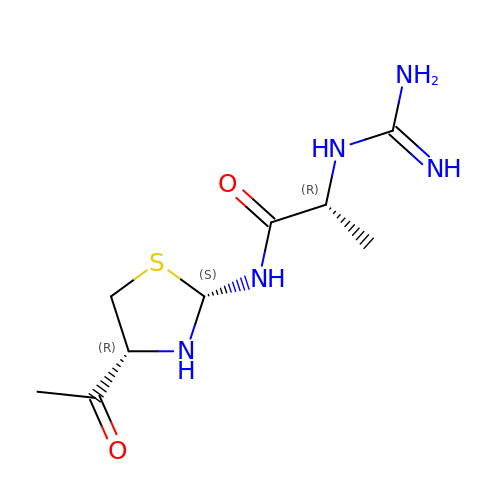(2~{R})-2-carbamimidamido-~{N}-(4-ethanoyl-1,3-thiazolidin-2-yl)propanamide | C9 H17 N5 O2 S | LAWADVQORXPDOH-VKJXWFFISA-N5,7-dimethylpyrazolo[1,5-a]pyrimidin-2-amine | C8 H10 N4 | 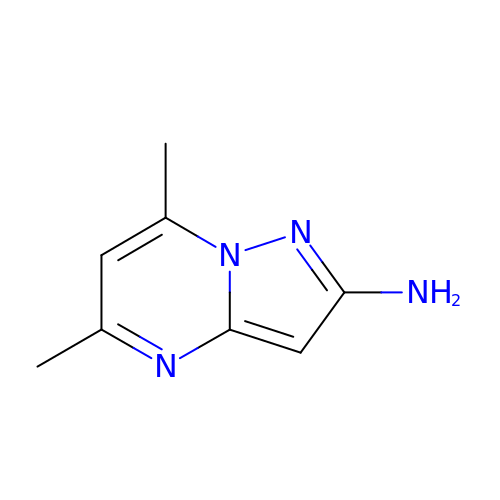JTTOBYJUZIFSFJ-UHFFFAOYSA-N>[2x]MRSRRVDVMDVMNRLILAMDLMNRDDALRVTGEVREYIDTVKIGYPLVLSEGMDIIAEFRKRFGCRIIADFKVADIPETNEKICRATFKAGADAIIVHGFPG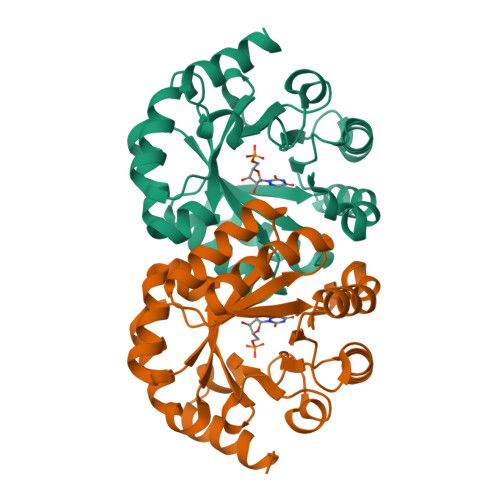ADSVRACLNVAEEMGREVFLLTEMPHPGAEMFIQGAADEIARMGVDLGVKNYVGPSTRPERLSRLREIIGQDSFLISPGVGAQGGDPGETLRFADAIIVGRSIYLADNPAAAAAGIIESIKDLLNP> MKVPPDVDPRYQKFLRQHVDADMSVQKCDRAMS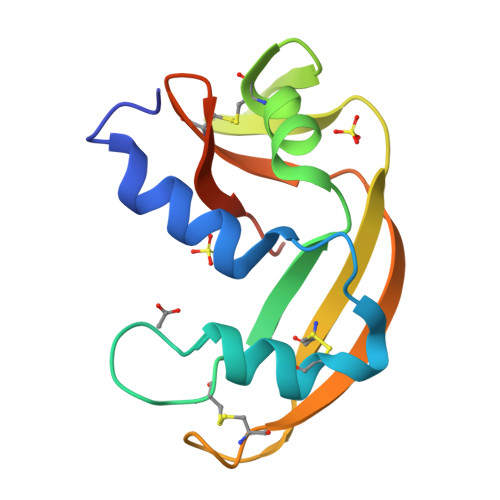IKKITAGTGNDCKEVNTFIQATKDRITTVCGDAGTPVNNLFKSNQPFPVVTCKLKSGNRRPNCQYRGTSSTRYIVLGCDKGWPVHYDEGIIDVNRSG>MAAIAFIGLGQMGSPMASNLLQQGHQLRVFDVNAEAVRHLVDKGATPAANPAQAAKDAEFIITMLPNGDLVRNVLFGENGVCEGLSTDALVIDMSTIHPLQTDKLIADMQAKGFSMMDVPVGRTSANAITGTLLLLAGGTAEQVERATPILMAMGSELINAGGPGMGIRVKLINNYMSIALNALSAEAAVLCEALNLPFDVAVKVMSGTAAGKGHFTTSWPNKVLSGDLSPAFMIDLAHKDLGIALDVANQLHVPMPLGAASREV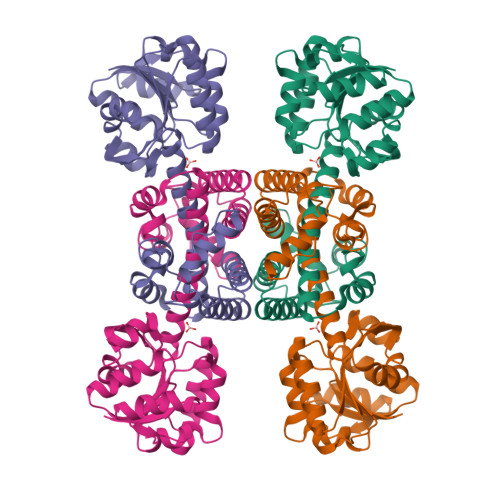YSQARAAGRGRQDWSAILEQVRVSAGMTAKVKMLEHHHHHH[4x]> AGSGHMDPDFLYRWALIGLAAFGAFSFATLFFVPAPYGRHQRGGWGPTVPTRLAWIAQELPAPLVFALVFARGEHADRLVPLLLLGLWQLHYLQRTFVFPLLMRVGAKRTPLVTALLAFVFNCVNGAANAYAITHGALRHTEA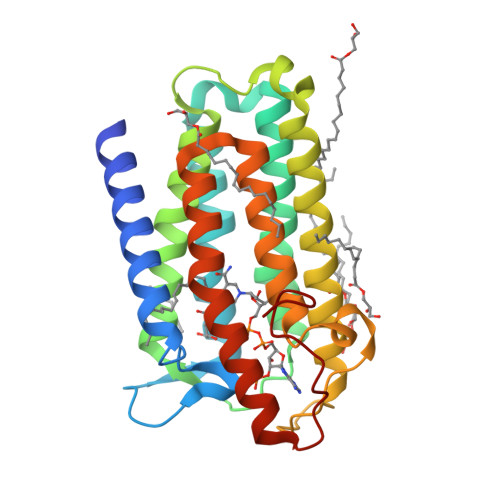WLADPRFAIGALLFLGGWALNLHSDAILRRLRAPGETRYEIPRGGAYRLVSCPNYLGEIVEWCGWALATWTYAGAVFAFFTFANLFPRALAHHRWYRERFPDYPRERKAVIPFVV>MKNKLVVVTGVPGVGGTTITQKAME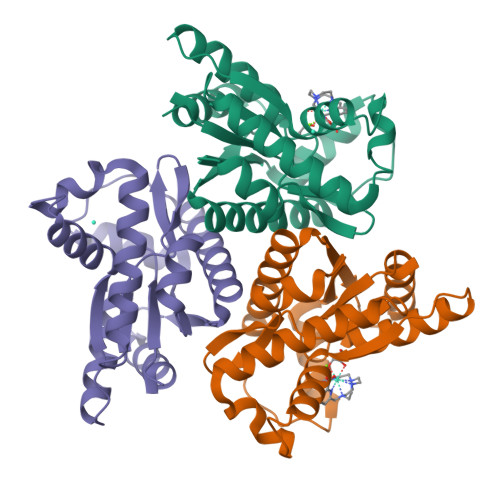KLSEEGINYKMVNFGTVMFEVAQEENLVEDRDQMRKLDPDTQKRIQKLAGRKIAEMVKESPVVVDTHSTIKTPKGYLPGLPVWVLNELNPDIIIVVETSGDEILIRRLNDETRNRDLETTAGIEEHQIMNRAAAMTYGVLTGATVKIIQNKNNLLDYAVEELISVLR[3x]Cyclic GMP-AMP synthase (cGAS) is the most recently identified member of the family of cytosolic DNA sensors. Cytosolic cGAS binds dsDNA and in the presence of ATP and GTP catalyzes the production of the recently characterized second messenger 2′, 3′- cyclic AMP-GMP (cGAMP) which then binds to Stimulator of Interferon Genes (STING). In humans, the binding of the cGAS product to STING causes a conformational change resulting in recruitment of TBK1, and interferon-inducible gene activation and interferon production via IRF3 phosphorylation and nuclear translocation. Activation of cGAS is important in host defense against pathogens, but uncontrolled activation of the cGAS pathway has been implicated in autoinflammatory disease.

The evidence linking activation of the cGAS pathway to autoimmune disease suggests that cGAS inhibitors may have therapeutic efficacy. Structure-based drug design and chemical optimization of the original fragment hit resulted in a high affinity lead that binds in the nucleotide binding site and inhibits cGAS activity. Taken together our results demonstrate the druggability of cGAS, provide a high affinity active site inhibitor and establish a sensitive screening assay with broad utility for cGAS drug discovery.

>GASKLRAVLEKLKLSRDDISTAAGMVKGVVDHLLLRLKCDSAFRGVGLLNTGSYYEHVKISAPNEFDVMFKLEVPRIQLEEYSNTRAYYFVKFKRNPKENPLSQFLEGEILSASKMLSKFRKIIKEEINDIKDTDVIMKRKRGGSPAVTLLISEKISVDITLALESKSSWPASTQEGLRIQNWLSAKVRKQLRLKPFYLVPKHAKEGNGFQEETWRLSFSHIEKEILNNHGKSKTCCENKEEKCCRKDCLKLMKYLLEQLKERFKDKKHLDKFSSYHVKTAFFHVCTQNPQDSQWDRKDLGLCFDNCVTYFLQCLRTEKLENYFIPEFNLFSSNLIDKRSKEFLTKQIEYERNNEFPVFDEF[2x]> MSNVQTSAEREIVDLSHLAFDCGMLGRLKTVSWTPVIAGDSFELDAVGALRLSPLRRGLAIDSKVDFFTFYIPHRHVYGDQWIQFMRDGVNAQPLPSVTCNRY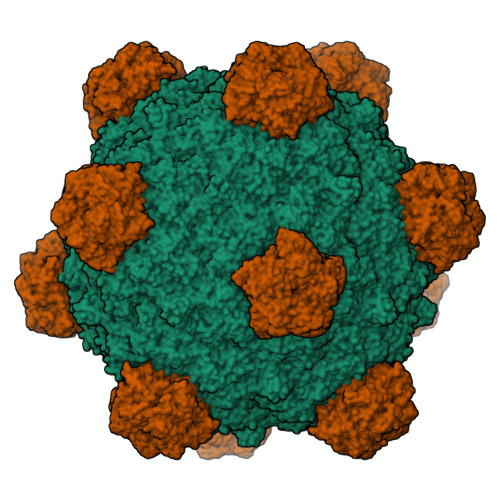PDHAGYVGTIVPANNRIPKFLHQSYLNIYNNYFRAPWMPERTEANPSNLNEDDARYGFRCCHLKNIWSAPLPPETKLAEEMGIESNSIDIMGLQAAYAQLHTEQERTYFMQRYRDVISSFGGSTSYDADNRPLLVMHTDFWASGYDVDGTDQSSLGQFSGRVQQTFKHSVPRFFVPEHGVMMTLALIRFPPISPLEHHYLAGKSQLTYTDLAGDPALIGNLPPREISYRDLFRDGRSGIKIKVAESIWYRTHPDYVNFKYHDLHGFPFLDDAPGTSTGDNLQEAILVRHQDYDACFQSQQLLQWNKQARYNVSVYRHMPTVRDSIMTS;> MYQNFVTKHDTAIQTSRFSVTGNVIPAAPTGNIPVINGGSITAERAVVNLYANMNVSTSSDGSFIVAMKVDTSPTDPNCVISAGVNLSFAGTSYPIVGIVRFESASEQPTSIAGSEVEHYPIEMSVGSGGVCSARDCATVDIHPRTSGNNVFVGVICSSAKWTSGRVIGTIATTQVIHEYQVLQPLK;> SKGKKRSGARPGRPQPLRGTKGKRKGARLWYVGGQQF>[2x]MDTVTGLPNRQLFCDRLLQALAAHERDGNPVVLLFLDVDNFKSINDSLGHLVGDRLLRATAERIRTAVRDGDTVARIGGDKFTILLNGAKDT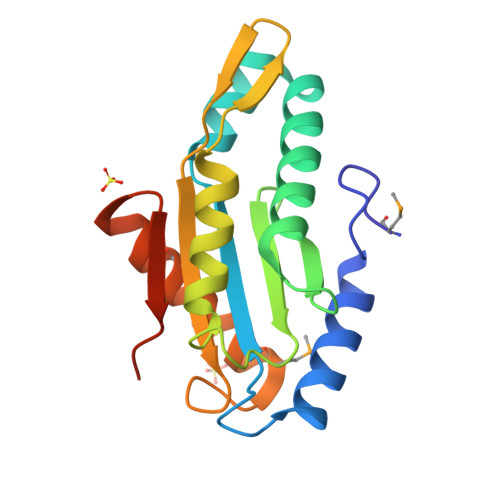LNGALVAQKILDGLAQPFVFGAQQIVISVSIGIAVSPADGETMEQLLRNADTAMYHAKSRGKNNYQFFSPELEHHHHHH> QKSSELVIGGNECDTNEHRFLAAFFTSRPWTFQCAGTLIHEEWVLAAAHCYKRGLNIYLGMHNQSIQFDDEQRRYAIEEHYYRCDEKLTKWEKDVVLLKLNKPVSNSTHIAPLSLPSSPPSIGSVCRVMGWGIMSSTKDILPDVPHCANINLLNYMECVAHYPDVPETTRLLCAGVLEGGIDTCNQDSGGPLICDGQF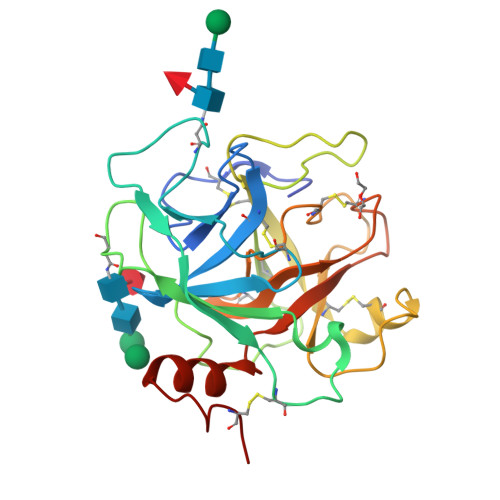QGIVFFGKYPCAQPNKPGLYTRVSNYNDWIQNIIAGKTTTACPP> EADRPKKVLILMSDTGGGHRASAEAIRAAFNQEFGDEYQVFITDLWTDHTPWPFNQLPRSYNFLVKHGTLWKMTYYGTSPRIVHQSNFAATSTFIAREIAQGLMKYQPDIIISVHPLMQHVPLRVLRSKGLLKKIVFTTVITDLSTCHPTWFHKLVTRCYCPSTEVAKRAQKAGLETSQIKVYGLPVRPSFVKPVRPKVELRRELGMDENLPAVLLMGGGEGMGPIEATARALADALYDKNLGEAVGQVLIICGRNKKLQSKLSSLDWKIPVQVKGFITKMEECMGACDCIITKAGPGTIAEAMIRGLPIILNGYIAGQEAGNVPYVVENGCG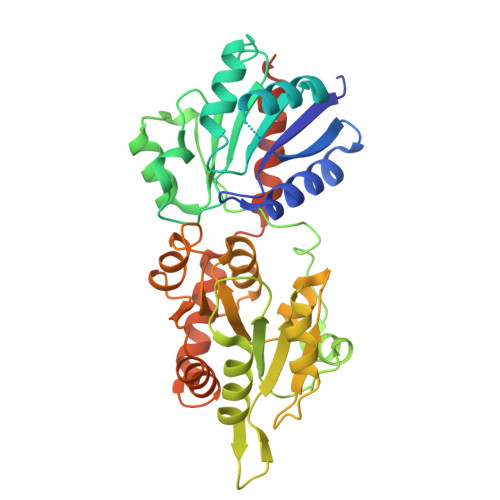KFSKSPKEISKIVADWFGPASKELEIMSQNALRLAKPEAVFKIVHDMHELVRKKNSLPQLSCTAAAALEHHHHHH> MTEKEKMLAEKWYDANFDQTLINERLRAKVICFALNHTNPSA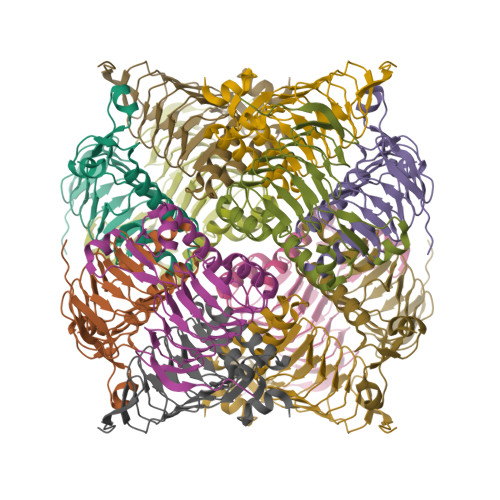TLKRKVLIDALFQTTTDNVSISIPFDTDYGWNVKLGKNVYVNTNCYFMDGGQITIGDNVFIGPNCGFYTATHPLNFHHRNEGFEKAGPIHIGSNTWFGGHVAVLPGVTIGEGSVIGAGSVVTKDIPPHSLAVGNPCKVVRKIDNDLPSETLNDETIKLEHHHHHH> GVQPLATQCFQLSNMFNPQTEEEVGWDTEIKDDVIEECNKHGGVIH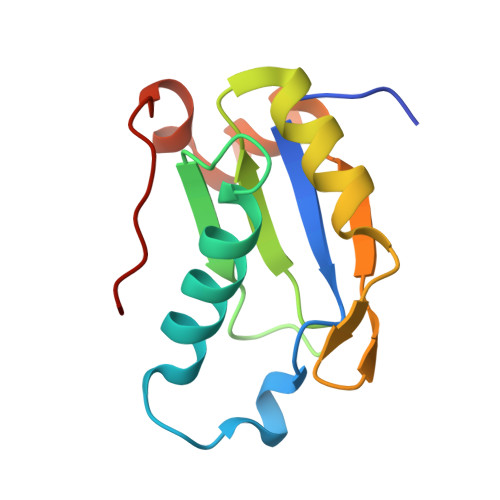IYVDKYSAQGNVYVKCPSIAAAIAAVNALHGRWFAGKMITAAYVPLPTYHNLFPDSMTATQLLVPSRR>MNPNQKIITIGSVCMTIGMANLILQIGNIISIWISHSIQLGNQNQIETCNQSVITYENNTWVNQTYVNISNTNFAAGQSVVSVKLAGNSSLCPVSGWAIYSKDNSIRIGSKGDVFVIREPFISCSPLECRTFFLTQGALLNDKHSNGTIKDRSPYRTLMSCPIGEVPSPYNSRFESVAWSASACHDGINWLTIGISGPDNGAVAVLKYNGIITDTIKSWRNNRLRTQESECACVNGSCFTVMTDGPSDGQASYKIFRIEKGKIVKSVEMNAPNYHYEECSCYPDSSEITCVCRDNWHGSNRPWVSFNQNLEYQIGYICSGIFGDNPRPNDKTGSCGPVSSNGANGVKGFSFKYGNGVWIGRTKSISSRNGFEMIWDPNGWTGTDNDFSIKQDIVGINEWSGYSGSFVQHPELTGLDCIRPCFWVELIRGRPKENTIWTSGSSISFCGVNSDTVGWSWPDGAELPFTIDK[2x]

Stimulated by the first neuraminidase (NA) crystal structures, the NAIs were designed to interact with the active site of all NA types. We identified a novel isoleucine to arginine change at position 223 (I223R) in the NA of a virus isolated from an immune suppressed child on prolonged oseltamivir and zanamivir therapy. In contrast to the frequently observed H275Y change, which causes selective resistance to oseltamivir, the I223R mutation conferred a resistance phenotype against both oseltamivir and zanamivir. Our results support this suggestion by indicating that a ligand-free form of the pandemic neuraminidase adopts an open conformation. Together with this structure we present the structures of the I223R mutant neuraminidase in complex with oseltamivir and zanamivir to investigate the resistance mechanism of the I223R mutant neuraminidase.

The first striking feature from these data is that the 150-loop in the ligand-free I223R NA adopts an open conformation, as seen in the first reported N1 structure, but in contrast to the closed conformation of this loop seen in the recently reported crystal structure of the 2009 pandemic A/H1N1 NA. Recent NMR experiments likely clarify the apparent discrepancy in these different studies by showing that the 150-loop is flexible and that an equilibrium between the open and closed conformations exists in solution. Inspection of our current structure shows that a phosphate ion, from the crystallization buffer, interacts with lysine 150 to stabilize the open conformation. We speculate that the different crystallization conditions used in the previous pandemic N1 study led to the stabilization of the closed form. The open conformation of the 150-loop (residues 148–151) generates an additional cavity at the edge of the active site that we have previously called the 150-cavity, which we have suggested to be an additional target site for neuraminidase inhibitor design. In the wild type N1 neuraminidase structure, a small pocket, the “223-pocket”, also adjacent to the active site, but distinct from the 150-cavity, contains two water molecules. In the I223R neuraminidase, this pocket is occupied by the side chain of R223. In displacing the two water molecules seen in the wild-type structure, the arginine makes a hydrogen bond with the side chain of serine 247 (S247). As a result, the side chain of S247 adopts a different rotamer and is oriented towards the active site which enables it to make a second hydrogen bond with glutamic acid 277 (E277). These changes in the structure of the I223R neuraminidase result in shrinkage at the edge of the active site pocket that accommodates the hydrophobic pentoxyl group of oseltamivir.>[6x]MNYLNNIRIENPLTICYTNDVVKNFTANGLLSIGASPAMSEAPEEAEEFYKVAQALLINIGTLTAQNEQDIIAIAQTANEAGLPIVFDPVAVGASTYRKQFCKLLLKSAKVSVIKGNASEILALIDDTATMKGTDSDANLDAVTIAKKAYAIYKTAIVITGKEDVIVQGDKAIVLANGSPLLARVTGAGCLLGGIIAGFLFRETEPDIEALIEAVSVFNIAAEVAAENENCGGPGTFSPLLLDTLYHLNETTYQQRIRIQEVEENLYFQSGHHHHHH

Here we report a detailed structure-function analysis of the kinase ThiM, which phosphorylates THZ in one of the first steps in vitamin B1 biosynthetic pathway. The quaternary structure of SaThiM is a triangular homo-trimer with dimensions of approximately 72 Å on a side and 47 Å thick with three independent active sites, each located within interface regions between two monomers. The following β-sheet strand 7 is antiparallel to strand 6 and following β-sheet strand 8, which is antiparallelly flanked by β-sheet strand 9. This fold of the phosphotransferase ThiM is homologous to that common to the group of ribokinase-like folded kinases. The three active sites, each located within the interface regions of two monomers respectively, are homologous to other known phosphoryl transfer ribokinase-like kinases.

Out of this in silico selected set of molecules, two were chosen as the most promising analogues for further investigations: 2-(1,3,5-Trimethyl-1H-pyrazol-4-yl) ethanol, hereinafter referred to as compound 1 (cpd 1) and 2-(2-Methyl-1H-imidazol-1-yl) ethanol referred to as compound 2 (cpd 2). The structures of these complexes could be refined to 1.87 Å and 1.62 Å resolution with R and Rfree values of 16.86% and 19.90% for the cpd 1 complex and R and Rfree values of 18.24% and 20.28% for the cpd 2 complex. The thiazole moiety was replaced by the non-sulfur containing heterocycles pyrazole and imidazole for cpd 1 and cpd 2, respectively. For both compounds the N3 is retained and a second nitrogen atom at position 2 and 5 is included in the heterocycle of cpd 1 and cpd 2 respectively. The overall coordination of the THZ analogue compounds in the active site regions of the ThiM trimer is remarkably comparable to that of the of natural substrate THZ. Both compounds form a H-bond to the amide nitrogen of amino acid M39 and show a similar orientation of their hydroxyethyl groups. The activity of ThiM was analyzed in vitro, as described in the methods section, showing that the specific activities of cpd 1 and cpd 2 are approximately 1.5 times higher compared to THZ, however show only 1/10 of the efficiency (kcat/KM) in comparison to the natural substrate THZ. The two novel compounds applied for co-crystallization in this study lack the thiazolium sulfur, present in the natural thiazolium moiety of thiamin, which is replaced by a carbon atom, supporting slightly higher flexibility in the active site in consequence of the reduced van der Waals radius. Cpd 2 has an additional nitrogen atom in the heterocycle and could, like cpd 1, undergo a TPP imino tautomerization after fusion with HMP. As a result this substance could be channeled via thiaminase (TenA) into the bacterial thiamin pool, where it could act as a thiamin antagonist equally potent as pyrithiamine.(9R,12R)-15-amino-12-hydroxy-6,12-dioxo-7,11,13-trioxa-12lambda~5~-phosphapentadecan-9-yl undecanoate | C22 H44 N O8 P | 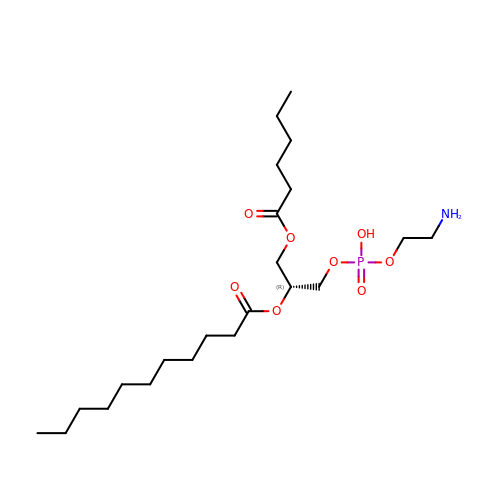WTEUZJKVOKXZKR-HXUWFJFHSA-N> EPQVLCYLTSWSSKRPSAGRFMPENVDPTLCTHVIYAFATLKDHKLTEADEKDADMYDKVVALREKNPNLKILLAIGGWAFGSTPFKELTSNVFRMNQFVYEAIEFLRDYQFNGLDVDWEYPRGADDRAAFVSLLKELRLAFEGEAKTSGQPRLLLTAAVPASFEAIAAGYDVPEISKYLDFINVMTYDFHGQWERQVGHNSPLFPLESATSYQKKLTVDYSAREWVRQGAPKEKLMIGMPTYGRSFTLINDTQFDIGAPASGGGQAGRFTNEAGFMSYYEICEFLREDNTTLVWDNEQMVPFAYREDQWVGFDDERSLKTKMAWLKEEGFGGIMVWSVDMDDFRGSCGTGKYPLITAMKQELSGYKVKLEYDGPYESSSPTGQYTTKDPHEVTCEEEDGHISYHKDHADCTMYYMCE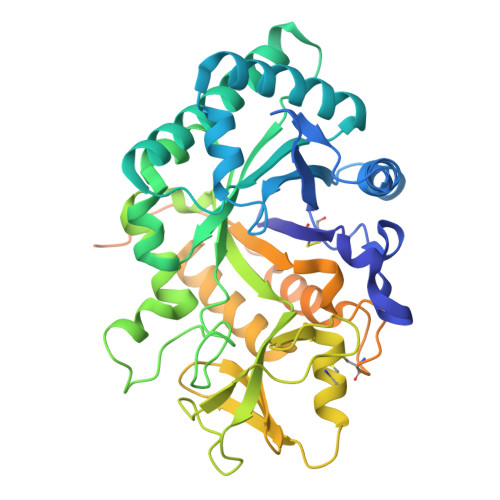GERKHHMPCPSNLVFNPNENVCDWPENVEGCQQHTQAPAAKR A library of known aspartic protease inhibitors was screened to identify compounds that inhibit plasmepsin V from Plasmodium vivax. This screen revealed compounds with an imino‐pyrimidinone‐fused pyrrolidine (IPF) scaffold that exhibited sub‐micromolar inhibitory activity against plasmepsin V. Further screening of IPF analogs against the related aspartic protease plasmepsin X showed inhibitory activity, while a third aspartic protease, plasmepsin IX, was not significantly inhibited.

Modifications to the P1 biaryl region of the IPF scaffold differentially modulated inhibition of both plasmepsin V and X. Notably, analogs with potent plasmepsin X inhibitory activity successfully blocked the growth of Plasmodium falciparum in vitro.

> GTHKVYKVGSEPIPCSQCKDVRECSACLFEEQDSPHAIHLKLNKKKPSDHSNLKKHHDSLKLGGVKYYVKRGEGISGSLGNPSGHTLDDIDSINEEIRIRREESAGVGRNGAEVTAYGGSGPSDRFAGVQRHAHAGGVSGDMASGEQRGSDEIAKGESFIDVKNAHAVVEQTEENVFLIPLKHLRDSQFVGTLLVGVPPQEIHPIFDTGSTNLWVVTTDCEEESCKKVKRYNPYKSKTFRRSFIGKNLHIVFGSGSISGSIGKETFVLGDHTVRNQTFGLVESESNDSLNGDNIFDYIDFEGIVGLGFPEMLSAGKVSFFDNLLSQNKNLSPQFSFYISPEDNTSTFLVGGVSKSFYEGSIYMLPVVKEYYWEVELDGIYVGEKKICCEEKSYAIFDTGTSYNTMPSAQMKGFFDVVPSAPCTEENYQEVLKNYPVIKYLFGDLVIELLPEEYMILNEESCIPAYMQIDVPSEKNHAYLLGSIAFMRHYYTVFVRGAGGQPSMVGVAKARAAAEAAQKVAELENLYFQGDYKDDDDKH>[10x]GWGQPHGGGWGQGGGTHSQWNK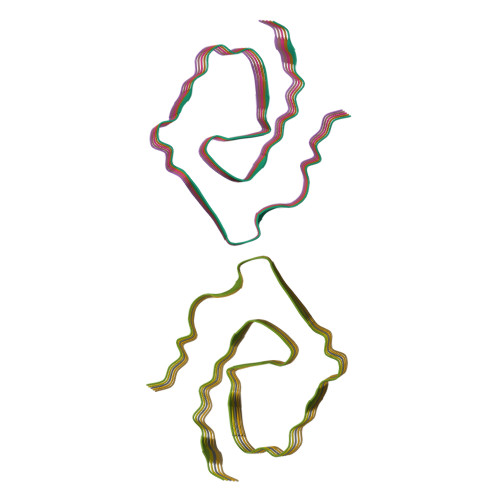PSKPKTNMKHMAGAAAAGAVVGGLGGYVLGSAMSRPIIHF~{N}-methyl-~{N}-[(1~{R})-1-pyridin-2-yl-3-pyrrolidin-1-yl-propyl]-5-[4,5,6,7-tetrakis(fluoranyl)-1~{H}-indol-3-yl]-1,3,4-oxadiazol-2-amine | C23 H22 F4 N6 O | 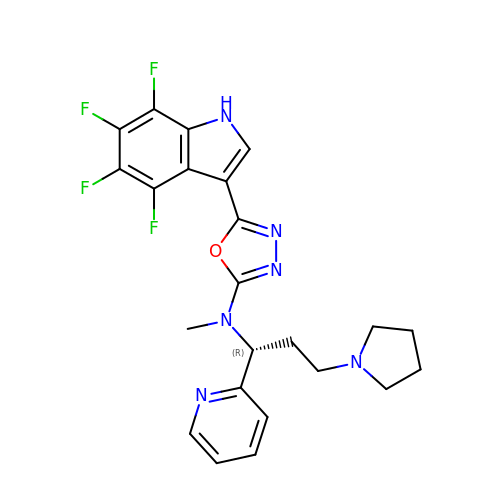IUWAZBMFUACYBK-OAHLLOKOSA-N>GPGSSLSRFRGCLAGALLGDCVGSFYAAHDTVDLTSVLRHVQSLEPDPGTPGSERTEALYYTDDTAMARALVQSLLAKEAFDEVDMAHRFAQEYKKDPDRGYGAGVVTVFKKLLNPKCRDVFEPARAQFNGKGSYGNGGAMRVAGISLAYSSVQDVQKFARLSAQLTHASSLGYNGAILQALAVHLALQGESSSEHFLKQLLGHMEDLEGDAQSVLDARELGMEERPYSSR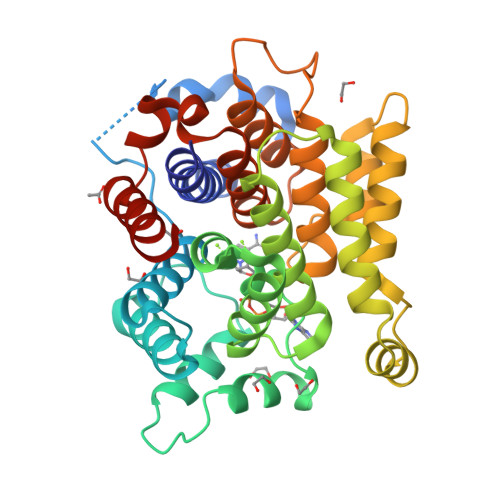LKKIGELLDQASVTREEVVSELGNGIAAFESVPTAIYCFLRCMEPDPEIPSAFNSLQRTLIYSISLGGDTDTIATMAGAIAGAYYGMDQVPESWQQSCEGYEETDILAQSLHRVFQKS[2x]> MASAATGVRAVPGNENSLEIEELARFAVDEHNKKENALLEFVRVVKAKEQVDLTRFPVTTMYYLTLEAKDGGKKKLYEAKVWVKGYLLEELKHNFKELQEFKPVGDAAAAHHHHHHHH;> MNNDHINLKVAGQDGSVVQFKIKRHTPLSKLMKAYCERQGL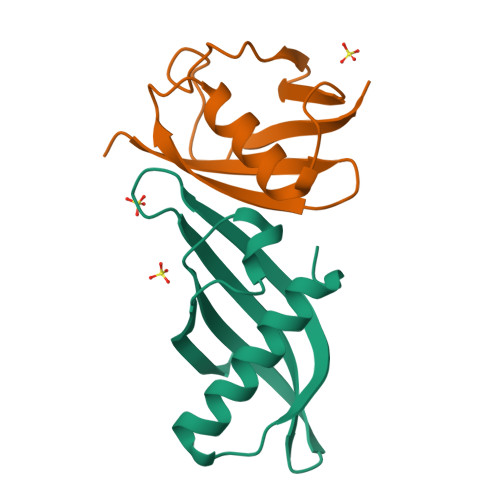SMRQIRFRFDGQPINETDTPAQLEMEDEDTIDVFQQ> MNARSTGQHPARYPGAAAGEPTLDSWQEPPHNRWAFAHLGEMVPSAAVSRRPVNAPGHALARLGAIAAQLPDLEQRLEQTYTDAFLVLRGTEVVAEYYRAGFAPDDRHLLMAVSKSLCGTVVGALVDEGRIDPAQ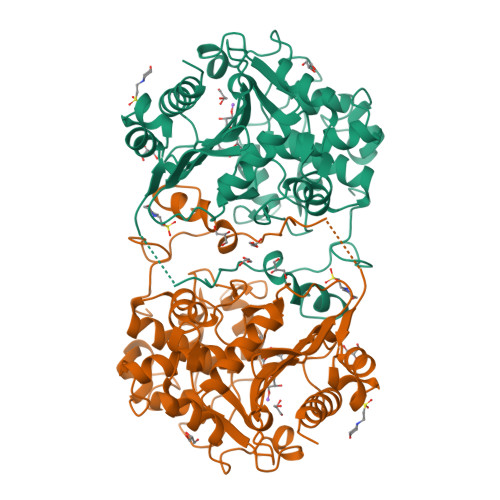PVTEYVPELAGSVYDGPSVLQVLDMQISIDYNEDYVDPASEVQTHDRSAGWRTRRHGDPADTYEFLTTLRGDGSTGEFQYCSANTDVLAWIVERVTGLRYVEALSTYLWAKLDADRDATITVDTTGFGFANGGVSCTARDLARVGRMMLDGGVAPGGRVVSEDWVRRVLAGGSHEAMTDKGFTNTFPDGSYTRQWWCTGNERGNVSGIGIHGQNLWLDPLTDSVIVKLSSWPDPYTEHWHRLQNGILLDVSRALDAV>[4x]GHMSTLLINQPQYAWLKELGLREENEGVYNGSWGGRGEVITTYCPANNEPIARVRQASVADYEETVKKAREAWKIWADIPAPKRGEIVRQIGDALREKIQVLGSLVSLEMGKILVEGVGEVQEYVDICDYAVGLSRMIGGPILPSERSGHALIEQWNPVGLVGIITAFNFPVAVYGWNNAIAMICGNVCLWKGAPTTSLISVAVTKIIAKVLEDNKLPGAICSLTCGGADIGTAMAKDERVNLLSFTGSTQVGKQVGLMVQERFGRSLLELGGNNAIIAFEDADLSLVVPSALFAAVGTAGQRCTTARRLFIHESIHDEVVNRLKKAYAQIR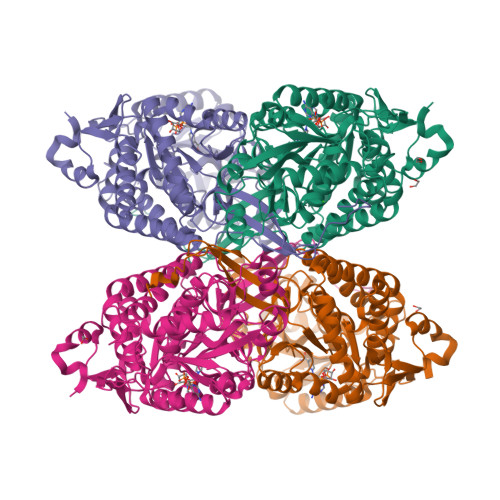VGNPWDPNVLYGPLHTKQAVSMFLGAVEEAKKEGGTVVYGGKVMDRPGNYVEPTIVTGLGHDASIAHTDTFAPILYVFKFKNEEEVFAWNNEVKQGLSSSIFTKDLGRIFRWLGPKGSDCGIVNVNIPTSGAEIGGAFGGEKHTGGGRESGSDAWKQYMRRSTCTINYSKDLPLAQGIKFQ> WDQMCIEKEANKTYNCENLGLSEIPDTLPNTTEFLEFSFNFLPTIHNRTFSRLMNLTFLDLTRCQINWIHEDTFQSHHQLSTLVLTGNPLIFMAETSLNGPKSLKHLFLIQTGISNLEFIPVHNLENLESLYLGSNHISSIKFPKDFPARNLKVLDFQNNAIHYISREDMRSLEQAINLSLNFNGNNVKGIELGAFDSTIFQSLNFGGTPNLSVIFNGLQNSTTQSLWLGTFEDIDDEDISSAMLKGLCEMSVESLNLQEH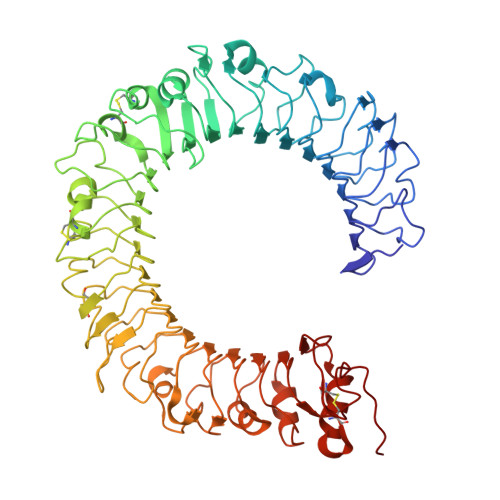RFSDISSTTFQCFTQLQELDLTATHLKGLPSGMKGLNLLKKLVLSVNHFDQLCQISAANFPSLTHLYIRGNVKKLHLGVGCLEKLGNLQTLDLSHNDIEASDCCSLQLKNLSHLQTLNLSHNEPLGLQSQAFKECPQLELLDLAFTRLHINAPQSPFQNLHFLQVLNLTYCFLDTSNQHLLAGLPVLRHLNLKGNHFQDGTITKTNLLQTVGSLEVLILSSCGLLSIDQQAFHSLGKMSHVDLSHNSLTCDSIDSLSHLKGIYLNLAANSINIISPRLLPILSQQSTINLSHNPLDCTCSNIHFLTWYKENLHKLEGSEETTCANPPSLRGVKLSDVKLSCG> MRVNNGLTPQELEAYGISDVHDIVYNPSYDLLYQEELDPSLTGYERGVLTNLGAVAVDTGIFTGRSPKDKYIVRDDTTRDTFWWADKGKGKNDNKPLSPETWQHLKGLVTRQLSGKRLFVVDAFCGANPDTRLSVRFITEVAWQAHFVKNMFIRPSDEELAGFKPDFIVMNGAKCTNPQWKEQGLNSENFVAFNLTERMQLIGGTWYGGEMIKGMVSMMNYLLPLKGIASMH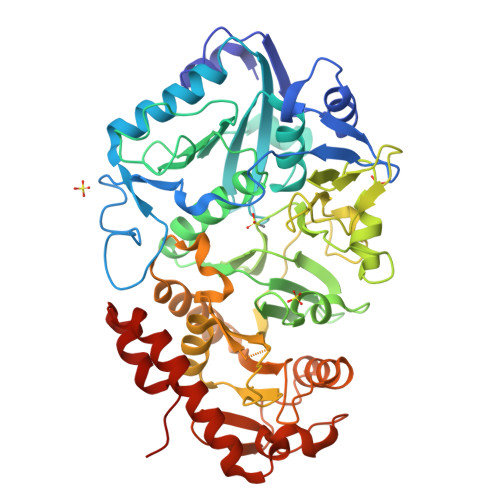CSANVGEKGDVAVFFGLSGTGKTTLSTDPKRRLIGDDEHGWDDDGVFNFEGGCYAKTIKLSKEAEPEIYNAIRRDALLENVTVREDGTIDFDDGSKTENTRVSYPIYHIDNIVKPVSKAGHATKVIFLTADAFGVLPPVSRLTADQTQYHFLSGFTAKLAGTERGITEPTPTFSACFGAAFLSLHPTQYAEVLVKRMQAAGAQAYLVNTGWNGTGKRISIKDTRAIIDAILNGSLDNAETFTLPMFNLAIPTELPGVDTKILDPRNTYASPEQWQEKAETLAKLFIDNFDKYTDTPAGAALVAAGPKLHHHHHH As a model β-strand mediated PPI, we use the GKAP/SHANK-PDZ50 which, plays a role in the organization of synaptic protein complexes and has been linked to several neuronal disorders. There are >250 PDZ domains with several therapeutically relevant proteins known to exhibit their function through a PDZ mediated interaction. Class I PDZ domains bind to consensus sequences with a Thr/Ser in the -2 position from the C-terminus, with the C-terminus hydrophobic residue and free carboxylate being the main determinants of affinity. Here, we used dynamic ligation screening to identify peptide-fragment hybrids linked through an acylhydrazone bond, that are able to functionally mimic a β-strand and inhibit its PPI using GKAP/SHANK1 PDZ as a model interaction.

In all hybrids, the hydrazone bond existed in an E configuration with the aromatic ring of the fragment co-planar with the hydrazone. The N terminal glutamate of the wild-type GKAP interacts with R679, thus we anticipated that the carboxylate of the hybrids might reproduce this same interaction. However, the N terminal part of the hybrids showed different binding behaviour in comparison with the wild type sequence. In some cases, we observed multiple conformations of the same compound having different orientations of the fragments relative to the peptide component presumably allowed by the conformational flexibility of the linker region. The more favourable entropy of binding supports the hypothesis that linker flexibility leads to a “fuzzier” mode of interaction (see below) although the carboxylate exhibited a slight preference for interaction with R736 (Fig. S19†) which differs from the wild-type GKAP peptide (see above) and likely arises from a combination of hybrid flexibility and the propensity of R736 to engage in effective charge-reinforced hydrogen-bonding interactions. Although this leads to slight uncertainty about the exact location of the fragments, we hypothesize that the key carboxylic acid moiety moves dynamically across a positively charged patch formed by R679, R736 and R743 on the protein surface, making transient charge-reinforced hydrogen-bonding and cation–π interactions which is also consistent with a more favourable entropy of interaction.

>GPLGSDYIIKEKTVLLQKKDSEGFGFVLRGAKAQTPIEEFTPTPAFPALQYLESVDEGGVAWRAGLRMGDFLIEVNGQNVVKVGHRQVVNMIRQGGNTLMVKVVMVTRHPDM[2x]>[2x]MSLEREEPQHFGAGPAQMPTPVLQQAAKDLINFNDIGLGIGEISHRSKDATKVIEDSKKHLIELLNIPDTHEVFYLQGGGTTGFSSVATNLAAAYVGKHGKIAPAGYLVTGSWSQKSFEEAKRLHVPAEVIFNAKDYNNGKFGKIPDESLWEDKIKGKAFSYVYLCENETVHGVEWPELPKCLVNDPNIEIVADLSSDILSRKIDVSQYGVIMAGAQKNIGLAGLTLYII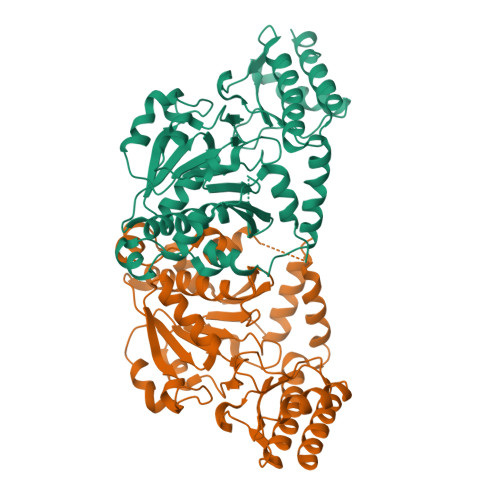KKSILKNISGASDETLHELGVPITPIAFDYPTVVKNNSAYNTIPIFTLHVMDLVFQHILKKGGVEAQQAENEEKAKILYEALDANSDFYNVPVDPKCRSKMNVVFTLKKDGLDDQFLKEAAARHLTGLKGHRSVGGFRASIYNALSVKAVQNLVDFIKEFAEKNA>STAAVAIRVAKKKLAKPPLDLHYLGDRVLRQPAKRVSRIDDELRQTIRQMLQTMYSADG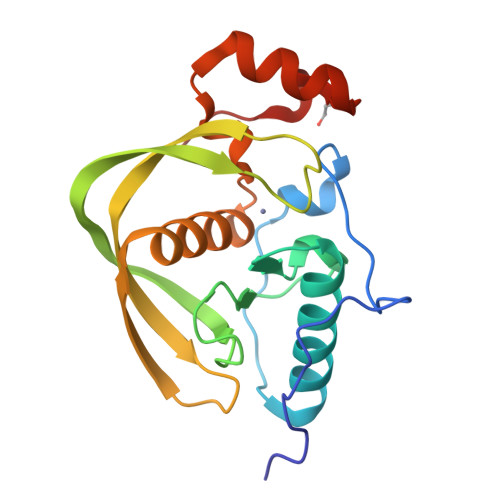IGLAAPQVGINKQLIVIDLELEDEQAPPLVLINPKIERTAGDLEQCQEGCLSIPGVYLDVERPEIVEVSYKDENGRPQRLVADGLLARCIQHEMDHLNGVLFVDRVENRLELNEALDKKGFAVQAVRPVAAAS[4x]> GSHMDVAGLTDCGLIRKSNQDAFYIDEKHQRFFIVADGMGGAAGGEEASRLAVDHIRQYLETHLEDLQHDPVTLLRQAFLAANHAIVEQQRQNSARADM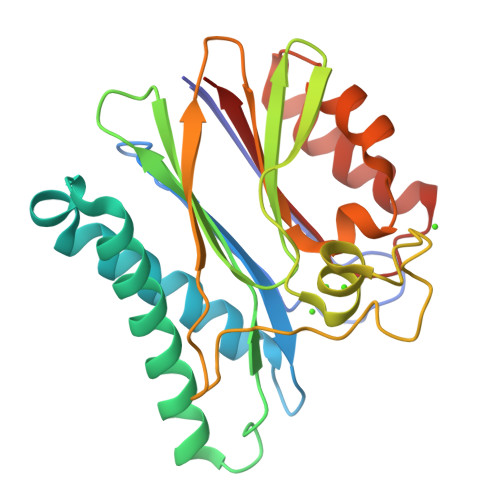GTTAVVILLDEKGDRAWCAHVGDSRIYRWRKDQLQQITSDHTWIAQAVQLGSLTIEQARQHPWRHVLSQCLGREDLSQIDIQPIDLEPGDRLLLCSDGLTEELTDDVISIYLSEPNVQKAAAALVDAAKTHGGRDNVTVVVISV>[2x]MSREEVESLIQEVLEVYPEKARKDRNKHLAVNDPAVTQSKKCIISNKKSQPGLMTIRGCAYAGSKGVVWGPIKDMIHISHGPVGCGQYSRAGRRNYYIGTTGVNAFVTMNFTSDFQEKDIVFGGDKKLAKLIDEVETLFPLNKGISVQSECPIGLIGDDIESVSKVKGAELSKTIVPVRCEGFRGVSQSLGHHIANDAVRDWVLGKRDEDTTFASTPYDVAIIGDYNIGGDAWSSRILLEEMGLRCVAQWSGDGSISEIELTPKVKLNLVHCYRSMNYISRHMEEKYGIPWMEYNFFGPTKTIESLRAIAAKFDESIQKKCEEVIAKYKPEWEAVVAKYRPRLEGKRVMLYIGGLRPRHVI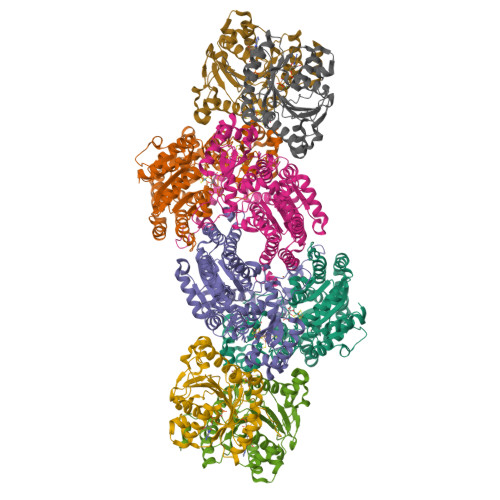GAYEDLGMEVVGTGYEFAHNDDYDRTMKEMGDSTLLYDDVTGYEFEEFVKRIKPDLIGSGIKEKFIFQKMGIPFRQMHSWDYSGPYHGFDGFAIFARDMDMTLNNPCWKKLQAPWE;>SQQVDKIKASYPLFLDQDYKDMLAKKRDGFEEKYPQDKIDEVFQWTTTKEYQELNFQREALTVNPAKACQPLGAVLCALGFEKTMPYVHGSQGCVAYFRSYFNRHFREPVSCVSDSMTEDAAVFGGQQNMKDGLQNCKATYKPDMIAVSTTCMAEVIGDDLNAFINNSKKEGFIPDEFPVPFAHTPSFVGSHVTGWDNMFEGIARYFTLKSMDDKVVGSNKKINIVPGFETYLGNFRVIKRMLSEMGVGYSLLSDPEEVLDTPADGQFRMYAGGTTQEEMKDAPNALNTVLLQPWHLEKTKKFVEGTWKHEVPKLNIPMGLDWTDEFLMKVSEISGQPIPASLTKERGRLVDMMTDSHTWLHGKRFALWGDPDFVMGLVKFLLELGCEPVHILCHNGNKRWKKAVDAILAASPYGKNATVYIGKDLWHLRSLVFTDKPDFMIGNSYGKFIQRDTLHKGKEFEVPLIRIGFPIFDRHHLHRSTTLGYEGAMQILTTLVNSILERLDEETRGMQATDYNHDLVR[2x];>[4x]AMRQCAIYGKGGIGKSTTTQNLVAALAEMGKKVMIVGCDPKADSTRLILHSKAQNTIMEMAAEAGTVEDLELEDVLKAGYGGVKCVESGGPEPGVGCAGRGVITAINFLEEEGAYEDDLDFVFYDVLGDVVCGGFAMPIRENKAQEIYIVCSGEMMAMYAANNISKGIVKYANSGSVRLGGLICNSRNTDREDELIIALANKLGTQMIHFVPRDNVVQRAEIRRMTVIEYDPKAKQADEYRALARKVVDNKLLVIPNPITMDELEELLMEFG>SAKDPMDRAAHAVEQWRSERPDLDPSSMIVLGRLQEAALVIARDRLNPLF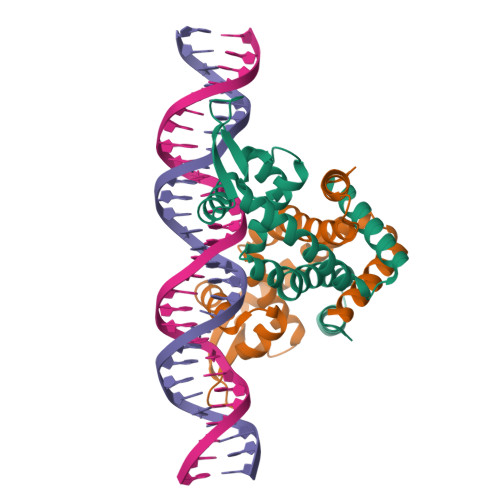ARYGLQPGEFDVLATLRRSGAPYALTPTALYDAAMISSGSMTNRIDRLEKAGWVERRANPADGRGTLVALTSAGRALIDDAVVAHVDNQRRVLSALSAAEQRQLAKLLDKLLQGQAAEG[2x]> MGKHHHHHHENLYFQGDEIYEDLMRSEPVSMPPKMTEYDKRCCCLREIQQTEEKYTDTLGSIQQHFLKPLQRFLKPQDIEIIFINIEDLLRVHTHFLKEMKEALGTPGAANLYQVFIKYKERFLVYGRYCSQVESASKHLDRVAAAREDVQMKLEECSQRANNGRFTLRDLLMVPMQRVLKYHLLLQELVKHTQEAMEKENLRLALDAMRDLAQCVNEVKRDNETLRQITNFQLSIENLDQSLAHYGR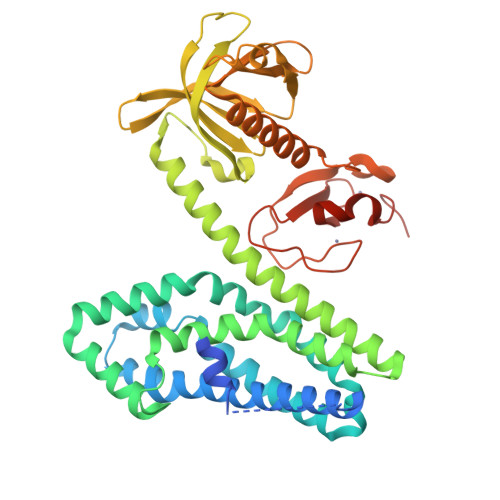PKIDGELKITSVERRSKMDRYAFLLDKALLICKRRGDSYDLKDFVNLHSFQVRDDSSGDRDNKKWSHMFLLIEDQGAQGYELFFKTRELKKKWMEQFEMAISNIYPENATANGHDFQMFSFEETTSCKACQMLLRGTFYQGYRCHRCRASAHKECLGRVPPCGRHGQDFPGTM>[6x]MTNTLQVRLLSENARMPERNHKTDAGYDIFSAETVVLEPQEKAVIKTDVAVSIPEGYVGLLTSRSGVSSKTHLVIETGKIDAGYHGNLGINIKNDA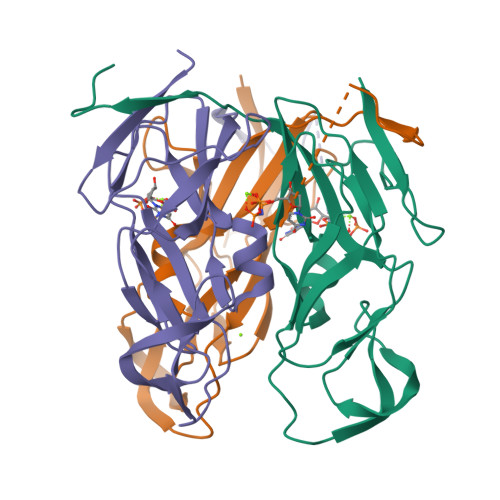IASNGYITPGVFDIKGEIDLSDAIRQYGTYQINEGDKLAQLVIVPIWTPELKQVEEFESVSERGEKGFGSSGV> SSLDDKPQFPGASAEFIDKLEFIQPNVISGIPIYRVMDRQGQIINPSEDPHLPKEKVLKLYKSMTLLNTMDRILYESQRQGRISFYMTNYGEEGTHVGSAAALDNTDLVFGQYREAGVLMYRDYPLELFMAQCYGNISDLGKGRQMPVHYGCKERHFVTISSPLATQIPQAVGAAYAAKRANANRVVICYFGEGAASEGDAHAGFNFAATLECPIIFFCRNNGYAISTPTSEQYRGDGIAARGPGYGIMSIRVDGNDVFAVYNATKEARRRAVAENQPFLIEAMTYRIGHHDTSDD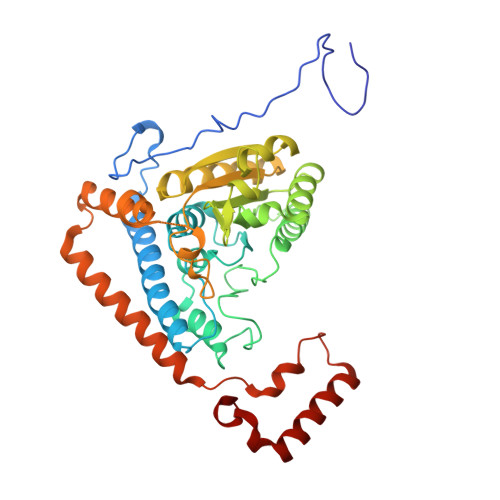SSAYRSVDEVNYWDKQDHPISRLRHYLLSQGWWDEEQEKAWRKQSRRKVMEAFEQAERKPKPNPNLLFSDVYQEMPAQLRKQQESLARHLQTYGEHYPLDHFDK> MSKFLDRFRYFKQKGETFADGHGQLLNTNRDWEDGYRQRWQHDKIVRSTHGVNCTGSCSWKIYVKNGLVTWETQQTDYPRTRPDLPNHEPRGCPSGASYSWYLYSANRLKYPMMRKRLMKMWREAKALHSDPVEAWASIIEDADKAKSFKQARGRGGFVRSSWQEVNELIAASNVYTIKNYGPDRVAGFSPIPAMSMVSYASGARYLSLIGGTCLSFYDWYCDLPPASPQTWGEQTDVPESADWYNSSYIIAWGSNVPQTRTPDAHFFTEVRYKGTKTVAVTPDYAEIAKLCDLWLAPKQGTDAAMALAMGHVMLREFHLDNPSQYFTDYVRRYTDMPMLVMLEERDGYYAAGRMLRAADLVDALGQENNPEWKTVAFNTNGEMVAPNGSIGFRWGEKGKWNLEQRDGKTGEETELQLSLLGSQDEIAEVGFPYFGGDGTEHFNKVELENVLLHKLPVKRLQLADGSTALVTTVYDLTLANYGLERGLNDVNCATSYDDVKAYTPAWAEQITGVSRSQIIRIAREFADNADKTHGRSMIIVGAGLNHWYHLDMNYRGLINMLIFCGCVGQSGGGWAHYVGQEKLRPQTGWQPLAFALDWQRPARHMNSTSYFYNHSSQWRYETVTAEELLSPMADKSRYTGHLIDFNVRAERMGWLPSAPQLGTNPLTIAGEAEKAGMNPVDYTVKSLKEGSIRFAAEQPENGKNHPRNLFIWRSNLLGSSGKGHEFMLKYLLGTEHGIQGKDLGQQGGVKPEEVDWQDNGLEGKLDLVVTLDFRLSSTCLYSDIILPTATWYEKDDMNTSDMHPFIHPLSAAVDPAWEAKSDWEIYKAIAKKFSEVCVGHLGKETDIVTLPIQHDSAAELAQPLDVKDWKKGECDLIPGKTAPHIMVVERDYPATYERFTSIGPLMEKIGNGGKGIAWNTQSEMDLLRKLNYTKAEGPAKGQPMLNTAIDAAEMILTLAPETNGQVAVKAWAALSEFTGRDHTHLALNKEDEKIRFRDIQAQPRKIISSPTWSGLEDEHVSYNAGYTNVHELIPWRTLSGRQQLYQDHQWMRDFGESLLVYRPPIDTRSVKEVIGQKSNGNQEKALNFLTPHQKWGIHSTYSDNLLMLTLGRGGPVVWLSEADAKDLGIADNDWIEVFNSNGALTARAVVSQRVPAGMTMMYHAQERIVNLPGSEITQQRGGIHNSVTRITPKPTHMIGGYAHLAYGFNYYGTVGSNRDEFVVVRKMKNIDWLDGEGNDQVQESVK;> MKIRSQVGMVLNLDKCIGCHTCSVTCKNVWTSREGVEYAWFNNVETKPGQGFPTDWENQEKYKGGWIRKINGKLQPRMGNRAMLLGKIFANPHLPGIDDYYEPFDFDYQNLHTAPEGSKSQPIARPRSLITGERMAKIEKGPNWEDDLGGEFDKLAKDKNFDNIQKAMYSQFENTFMMYLPRLCEHCLNPACVATCPSGAIYKREEDGIVLIDQDKCRGWRMCITGCPYKKIYFNWKSGKSEKCIFCYPRIEAGQPTVCSETCVGRIRYLGVLLYDADAIERAASTENEKDLYQRQLDVFLDPNDPKVIEQAIKDGIPLSVIEAAQQSPVYKMAMEWKLALPLHPEYRTLPMVWYVPPLSPIQSAADAGELGSNGILPDVESLRIPVQYLANLLTAGDTKPVLRALKRMLAMRHYKRAETVDGKVDTRALEEVGLTEAQAQEMYRYLAIANYEDRFVVPSSHRELAREAFPEKNGCGFTFGDGCHGSDTKFNLFNSRRIDAIDVTSKTEPHP;> MQFLNMFFFDIYPYIAGAVFLIGSWLRYDYGQYTWRAASSQMLDRKGMNLASNLFHIGILGIFVGHFFGMLTPHWMYEAWLPIEVKQKMAMFAGGASGVLCLIGGVLLLKRRLFSPRVRATTTGADILILSLLVIQCALGLLTIPFSAQHMDGSEMMKLVGWAQSVVTFHGGASQHLDGVAFIFRLHLVLGMTLFLLFPFSRLIHIWSVPVEYLT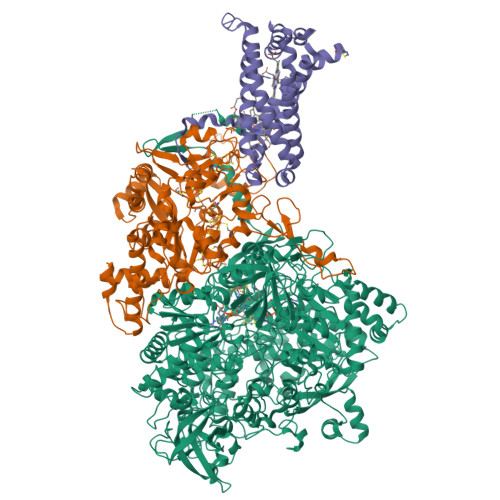RKYQLVRARH>[2x]AGGHGDVGMHVKEKEKNKDENKRKDEERNKTQEEHLKEIMKHIVKIEVKGEEAVKKEAAEKLLEKVPSDVLEMYKAIGGKIYIVDGDITKHISLEALSEDKKKIKDIYGKDALLHEHYVYAKEGYEPVLVIQSSEDYVENTEKALNVYYEIGKILSRDILSKINQPYQKFLDVLNTIKNASDSDGQDLLFTNQLKEHPTDFSVEFLEQNSNEVQEVFAKAFAYYIEPQHRDVLQLYAPEAFNYMDKFNEQEINLSLEELKDQRMLSRYEKWEKIKQHYQHWSDSLSEEGRGLLKKLQIPIEPKKDDIIHSLSQEEKELLKRIQIDSSDFLSTEEKEFLKKLQIDIRDSLSE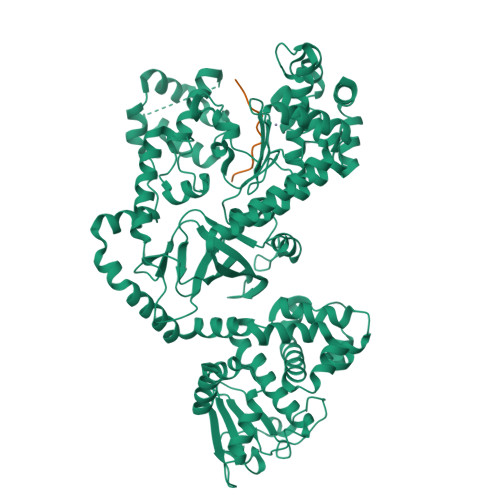EEKELLNRIQVDSSNPLSEKEKEFLKKLKLDIQPYDINQRLQDTGGLIDSPSINLDVRKQYKRDIQNIDALLHQSIGSTLYNKIYLYENMNINNLTATLGADLVDSTDNTKINRGIFNEFKKNFKYSISSNYMIVDINERPALDNERLKWRIQLSPDTRAGYLENGKLILQRNIGLEIKDVQIIKQSEKEYIRIDAKVVPKSKIDTKIQEAQLNINQEWNKALGLPKYTKLITFNVHNRYASNIVESAYLILNEWKNNIQSDLIKKVTNYLVDGNGRFVFTDITLPNIAEQYTHQDEIYEQVHSKGLYVPESRSILLHGPSKGVELRNDSEGFIHCFGHAVDDYAGYLLDKNQSDLVTNSKKFIDIFKEEGSNLTSYGRTNEAEFFAEAFRLMHSTDHAERLKVQKNAPKTFQFINDQIKFIINS;>MLARRKKVYPYPMEPTIAEG[2x]>VPALTREQLYIFDTTGFLVIPGVFGSGEVESFRSELERLDTVDPGFPRTRRYPDLPAASPVFARLALDDRLLAPVRDVVNQPLRLLEGYGLRRTKDSVLYLHGGNSELLDLGDRQVGRDLSITHTYHDGKLYCPYVKALVYLSD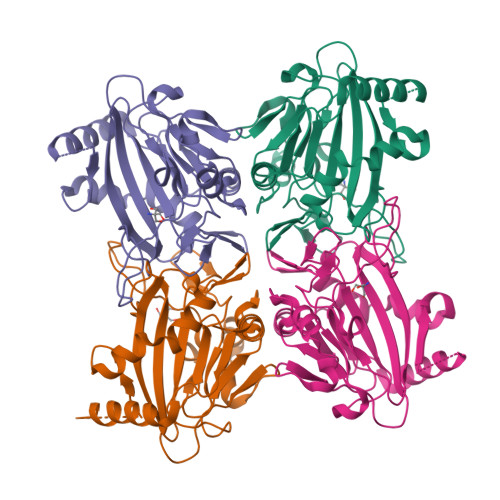IQSPEDGSFCYVQGSHKANFPLLRERAERGENTSLVDSGFPTLSDVFVRSGDVLLLNEALMHGTRRKLTEGDRLLTAFGYGPTFFTEWRELDAETADLRGAGYVDHDVEEDFVL[6x]(2S)-3-phenyl-2-[(3R)-pyrrolidin-3-yl]propanoic acid | C13 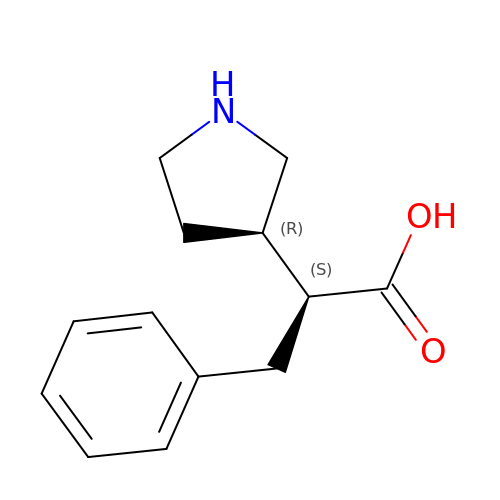H17 N O2 | OSTNIMGVYREMID-RYUDHWBXSA-N> GPLGSEAAPEYRVIVDANNLTVEIENELNIIHKFIRDKYSKRFPELESLVPNALDYIRTVKELGNSLDKCKNNENLQQILTNATIMVVSVTASTTQGQQLSEEELERLEEACDMALELNASKHRIYEYVESRMSFIAPNLSIIIGASTAAKIMGVAG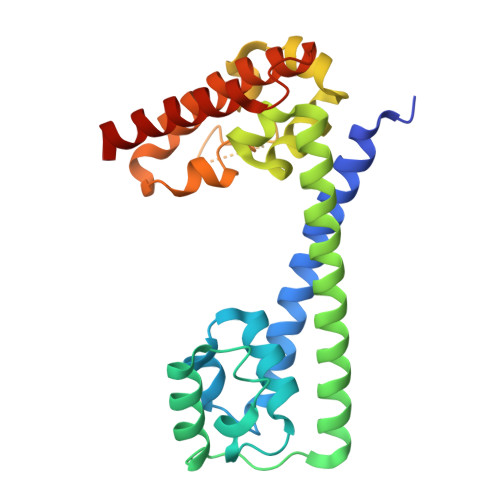GLTNLSKMPACNIMLLGAQRKTLSGFSSTSVLPHTGYIYHSDIVQSLPPDLRRKAARLVAAKCTLAARVDSFHESTEGKVGYELKDEIERKFDKWQE>[3x]MSTVVVKGNVNGGVQQPRMRRRQSLRRRANRVQPVVMVTAPGQPRRRRRRRGGNRRSRRTGVPRGRGSSETFVFTKDNLVGNTQGSFTFGPSLSDCPAFKDGILKAYHEYKITSILLQFVSEASSTSSGSIAYELDPHCKVSSLQSYVNKFQITKGGAKTYQARMINGVEWHDSSEDQCRILWKGNGKSSDSAGSFRVTIKVALQNPK

The Luteoviridae are an important family of pathogenic viruses responsible for necrosis of the plant vasculature which, in turn, causes severe stunting and dwarfism, and ultimately crop loss. The structures for BYDV and PLRV each reveal a luteovirid capsid composed of 180 CP monomers. The CP monomers each contain a single canonical jellyroll fold, and are arranged with T = 3 icosahedral quasi-symmetry to give a particle with a diameter of ∼30 nm. The luteovirid capsids are formed from CP subunits with a canonical jellyroll fold comprising two opposing β sheets, each containing 4 antiparallel β strands (βB-βI).

We therefore present high-resolution structures for VLPs of BYDV and PLRV at 3.0-Å and 3.4-Å resolution, respectively. BYDV and PLRV CPs assembled into monodisperse, homogeneous particles of the anticipated diameter. When imaged in ice, both BYDV and PLRV VLPs were monodisperse, so cryo-EM datasets were collected for each (see STAR Methods). Structure refinement was carried out with icosahedral symmetry imposed, yielding density maps at a resolution of 3.0 Å for BYDV and 3.4 Å for PLRV (see Table S1 for refinement statistics). Density maps for each structure were of sufficient quality and resolution to allow for unambiguous building of the shell (S) domain of the CP (BYDV: residues 61–200∗; PLRV: residues 68–208). In both cases the N-terminal R (RNA-binding) domain is not resolved in the cryo-EM density, except in the “C” conformer of BYDV, where an additional six residues of the R domain (residues 55–60) are visible. We have also solved the structure of VLPs formed by an N-terminally His-tagged version of PLRV CP to 3.4-Å resolution, since the formation of His-tagged VLPs were previously reported (Lamb et al., 1996). No differences were found between the structures of the VLPs formed by tagged and untagged CPs. For instance, mutations in the CP of PLRV that affect aphid transmission can now be rationalized (Kaplan et al., 2007). The triple mutant D95E, P97A, K100S had no impact upon capsid formation, but decreased transmission efficiency, suggesting that this region of the CP may be important for transmission. Our structures show that D95, P97, and K100 are situated within α1 and the preceding loop, and all three side chains are surface exposed, where they could, for example, affect binding of the virus to receptor(s) in the aphid vector.>[2x]MKQYLELMQKVLDEGTQKNDRTGTGTLSIFGHQMRFNLQDGFPLVTTKRCHLRSIIHELLWFLQGDTNIAYLHENNVTIWDEWADENGDLGPVYGKQWRAWPTPDGRHIDQITTVLNQLKNDPDSRRIIVSAWNVGELDKMAL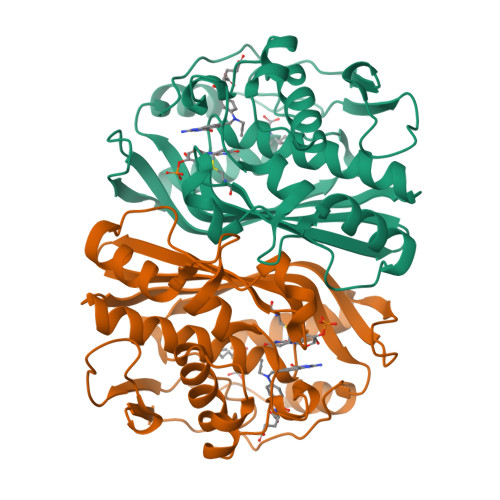APCHAFFQFYVADGKLSCQLYQRSCDVFLGLPFNIASYALLVHMMAQQCDLEVGDFVWTGGDTHLWSNHMDQTHLQLSREPRPLPKLIIKRKPESIFDYRFEDFEIEGYDPHPGIKAPVAI> ADNLAEFHVQNQECDSCHTPDGELSNDSLTYENTQCVSCHGTLAEVAETTKHEHYNAHASHFPGEVACTSCHSAHEKSMVYCDSCHSFDFNMPYAKKWLRDEPTIAELAKDKSERQAALASAPHDTVDVVVVGSGGAGFSAAISATDSGAKVILIEKEPVIGGNAKLAAGGMNAAWTDQQKAKKITDSPELMFEDTMKGGQNINDPALVKVLSSHSKDSVDWMTAMGADLTDVGMMGGASVNRAHRPTGGAGVGAHVVQVLYDNA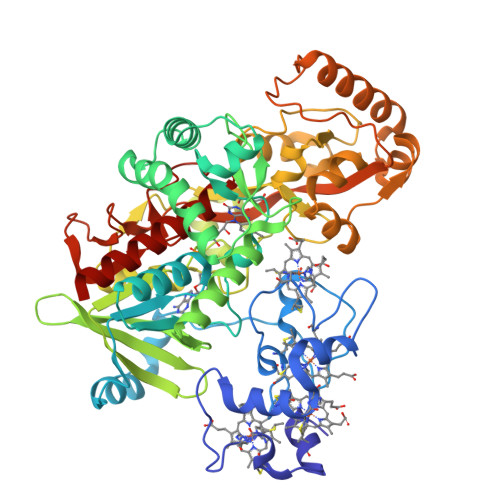VKRNIDLRMNTRGIEVLKDDKGTVKGILVKGMYKGYYWVKADAVILATGGFAKNNERVAKLDPSLKGFISTNQPGAVGDGLDVAENAGGALKDMQYIQAHPTLSVKGGVMVTEAVRGNGAILVNREGKRFVNEITTRDKASAAILAQTGKSAYLIFDDSVRKSLSKIDKYIGLGVAPTADSLVKLGKMEGIDGKALTETVARYNSLVSSGKDTDFERPNLPRALNEGNYYAIEVTPGVHHTMGGVMIDTKAEVMNAKKQVIPGLYGAGEVTGGVHGANRLGGNAISDIITFGRLAGEEAAKYSKKN ADENYLYL-3'-5'-PHOSPHO-URIDINE-3'-MONOPHOSPHATE 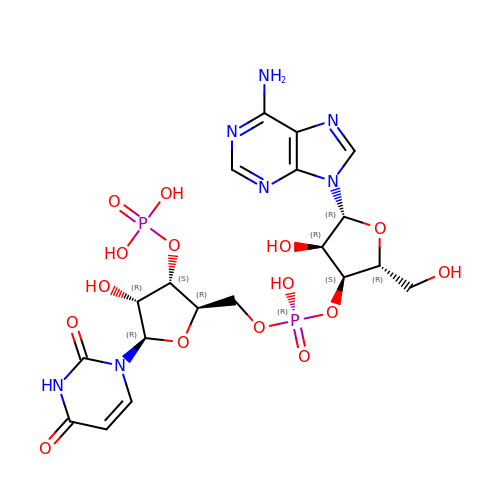| C19 H25 N7 O15 P2 | FZCSEXOMUJFOHQ-KPKSGTNCSA-N>[2x]GPLGSMNVSIEEFTHFDFQLVPEPSPLDLVITESLKNHIEVNGVKSGALLPLPFQTGIGKTYTALNFLLQQMLEQVRSELKEENTGKKSKRLLYYVTDSVDNVVSAKADLLKLIEKQTVKGEPRFTLEQQEYLKAQIVHLPNQSEQLLQCSDAVLNDVLIGFNLNAERDVQAEWSAISGLRRHASNPEVKISLNRQAGYFYRNLIDRLQKKQKGADRVLLSGSLLASVETLLPGEKIRNGSAHVAFLTTSKFLKGFHNTRSRYSPLRDLSGAVLIIDEIDKQNQVILSELCKQQAQDLIWAIRTLRANFRDHQLESSPRYDKIEDLFEPLRERLEEFGTNWNLAFAFNTEGANLNERPVRLFSDRSFTHVSSATHKLSLKSDFLRRKNLIFSDEKVEGSLIEKHGLLTRFVNEADVIYQWFLGTMRK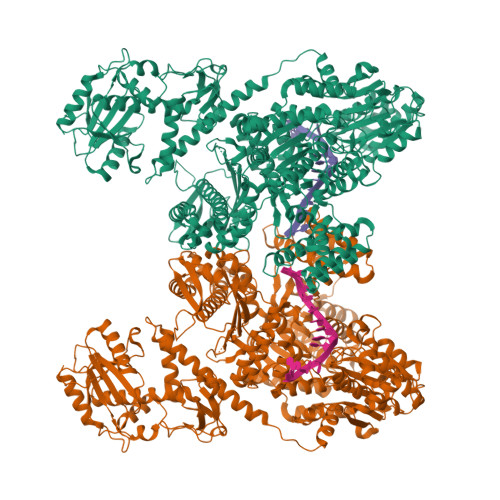AVFQYWENVRGLEIEVRENRSLEGTFQEAVQSLLTHFNLQEFESAVYESFDTRGLRQSAGGKANKLSSSKSYHHTGLKLVEVAHNQGTRDTVNCKASFLNTSPSGVLADMVDAGAVILGISATARADTVIHNFDFKYLNERLGNKLLSLSREQKQRVNNYYHSRRNYKDNGVVLTVKYLNSRDAFLDALLEEYKPEARSSHFILNHYLGIAESEQAFVRSWLSKLLASIKAFISSPDNRYMLSLLNRTLDTTRQNINDFIQFCCDKWAKEFNVKTKTFFGVNADWMRLVGYDEISKHLNTELGKVVVFSTYASMGAGKNPDYAVNLALEGESLISVADVTYSTQLRSDIDSIYLEKPTQLLLSDDYSHTANQLCQFHQILSLQENGELSPKSAENWCRQQLMGMSRERSLQQYHQTSDYQSAVRKYIEQAVGRAGRTSLKRKQILLFVDSGLKEILAEESRDPSLFSHEYVALVNKAKSAGKSIVEDRAVRRLFNLAQRNNKDGMLSIKALVHRLHNQPASKSDIQEWQDIRTQLLRYPTVAFQPERFNRLYLQSMTKGYYRYQGNLDGDPNSFEFFDRVPYGDMVSEEDCSLATLVQNQYVRPWFERKGFACSWQKEANVMTPIMFTNIYKGALGEQAVEAVLTAFDFTFEEVPNSIYERFDNRVIFAGIEQPIWLDSKYWKHEGNESSEGYSSKIALVEEEFGPSKFIYVNALGDTSKPIRYLNSCFVETSPQLAKVIEIPALIDDSNADTNRTAVQELIKWLHHS>[2x]GSPHMTKAEKILARFNELPNYDLKAVCTGCFHDGFNEVDIEILNQLGIKIFDNIKETDKLNCIFAPKILRTEKFLKSLSFEPLKFALKPEFIIDLLKQIHSKKDKLSQININLFDYEINGINESIISKTK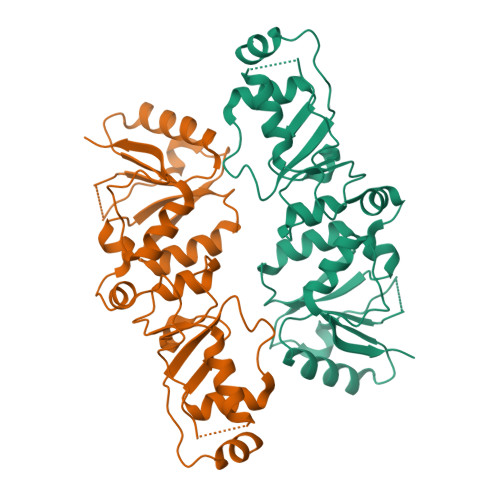LPTKVFERANIRCINLVNDIPGGVDTIGSVLKAHGIEKINVLRSKKCTFEDIIPNDVSKQENGGIFKYVLIVTKASQVKKFTKLINDRDKNETILIVEWNWCVESIFHLNVDFTSKKNVLYQKKNN> MHHHHHHE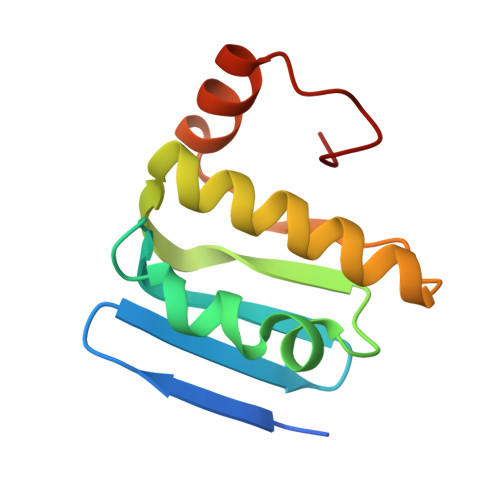NLYFQSESLSWMQTGDTLALSGELDQDVLLPLWEMREEAVKGITCIDLSRVSRVDTGGLALLLHLIDLAKKQGNNVTLQGVNDKVYTLAKLYNLPADVLPR Here, we describe the discovery that class I terpene cyclases are bifunctional, in that they catalyze both terpene cyclization and aromatic prenyltransferase reactions in the same active site. Class I terpene cyclases require 3 Mg2+ ions for catalytic function, and these metal ions are coordinated by conserved metal-binding motifs in a unique α-helical protein fold. Interestingly, the diterpene synthase FgGS can accept GPP as substrate donor to produce long-chain prenylindoles 11–14. Compounds 11 and 14 were characterized as previously reported (E)-1-(3,7-dimethylocta-2,6-dien-1-yl)-1H-indole and (E)-3-(3,7-dimethylocta-2,6-dien-1-yl)-1H-indole, respectively. This characterization implies that the active site cavity of FgGS is sufficiently large to allow the binding of indole as well as C5 DMAPP or C10 GPP to produce prenylindoles.

The crystal structure of FgGS complexed with Mg2+3-PPi and imidazole was determined at 2.15 Å resolution. The protein structure in this complex is essentially identical to that in the BTAC complex (rms deviation = 0.15 Å for 292 Cα atoms in monomer A). Metal coordination and hydrogen bond interactions for the PPi group in this complex are identical to those observed in the BTAC complex. Unexpectedly, imidazole and not indole is trapped in the active site of this structure. Imidazole was required for crystallization and the concentrations of imidazole and indole were 50 mM and 1 mM, respectively. Therefore, imidazole out-competed indole for binding in the active site during crystallization. Intermolecular interactions suggest that imidazole is bound as the positively charged imidazolium cation. The imidazolium N2-H group donates a hydrogen bond to the bridging oxygen of PPi, and the imidazolium N1-H group donates a hydrogen bond to a water molecule (monomer A) or ethylene glycol (monomer B). While all side chains of both complexes are in approximately the same position in the active site, R216 of the FgGS–Mg2+3–PPi–imidazole complex in monomer A adopts two conformations.

>MDPYSETSDLVDISRFDTHGLGANYKLRRHKFEHLADTGCHKARSDWVKYIGPLTEFGGCNHINGNFSAVVLPLCRPDRLELIAYVLEFAFLHDSVLESENTSPESEVQAEAGLRLLYERCISRLLQTDEVCAKKIAKTWKDAINTTTKDKNVDFQSIEDYLEFRMIDTGAPFVEALMLFGLGMSLSPQEDDALGHVIRPCFAALALTNDYFSFDREIEEVDTSTLINSVAIVMRIQSLDIPTAKTIINETIQKYEREFLRRIDEYKQHKGPISNKIEQYMEAMTYQISGNLVWSLNCPRYNPDYRYGLEACQHEG[2x]>[2x]GGGGU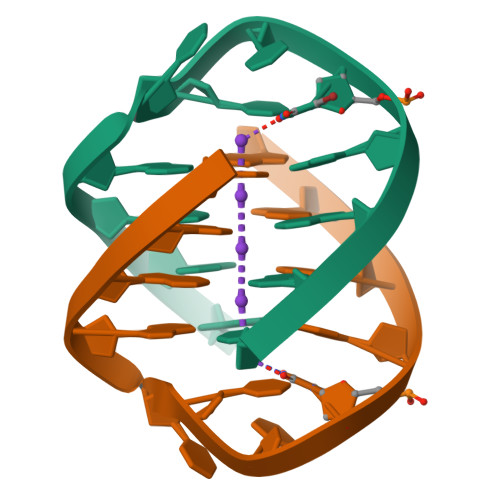TTTGGGG>[10x]ARILEDSPNARINKTILDRYLSLPLQENIVQATYVWIDGTGED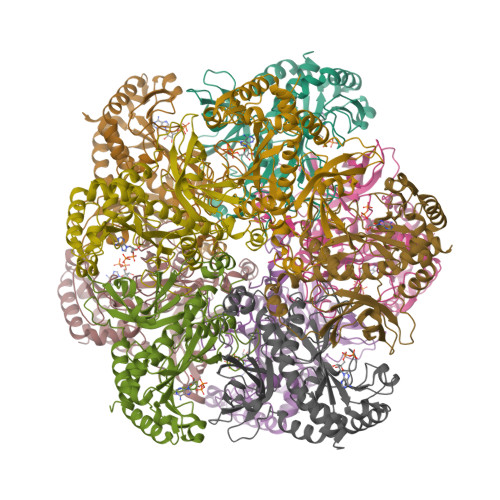LRCKDRTLDFIPQSPKELPVWNYDGSSCYQAEGSNSDTYLYPVAIYKDPFRRGNNILVMCDTYKFDGTPTDTNKRKTCLEVANKCAAEEPWFGIEQEYTFLDFDGHPLGWPKNGFPGPQGPYYCGVGANKVYARDIVDAHYRACLYAGIKVSGTNAEVMPAQWEFQVGPCEGISIGDDLWMARFLLHRISEEFGIVSTLDPKPMPGDWNGAGAHTNVSTKAMREDGGIRDIEKAVAKLSKCHERHIRAYDPKQGQDNARRLTGKHETSSINDFSAGVANRGCSIRIPRGVNDDGKGYFEDRRPSSNCDPYSVVEAILRTICLDE> MTAIRVCSRKFPTFASIFFQNITRNPSIHRISFSNLKPKTLLHPIPPKPFTVFVSRFHDGRPRGPLWRGKKLIGKEALFVILGLKRLKEDDEKLDKFIKTHVFRLLKLDMLAVIGELERQEETALAIKMFEVIQKQEWYQPDVFMYKDLIVSLAKSKRMDEAMALWEKMKKENLFPDS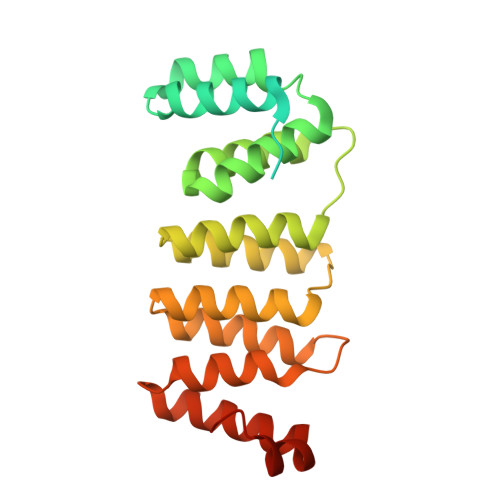QTYTEVIRGFLRDGCPADAMNVYEDMLKSPDPPEELPFRVLLKGLLPHPLLRNKVKKDFEELFPEKHAYDPPEEIFGRC> PGSMNELKHAVVPIDLQSFCLEGTLALWVPALENDSEDDSEAIETADDNEKLFKKECVAYDAGVYTSNKSKGSQTLRWSIFQNRTLTIFDVSLNSKKEPLSKFNVKIHFPSNVMKDGVAFSFSEHSDTTIIYAITHARVLYYIRLSKTWFQLPDARLDDDWCLCYRPISFLNQKPDLMAAISTSEICVSFFNGGLTKIILNPKDASHYEQHIDDSSYLFSLKKYLSLQAFKADYRSPNTIISMIFLSTYNVLVMLSLDYKLKVLDLSTNQCVETIELSQTILPLQSFPYLTSDHTTNSFIALYYPDNSHGSFSIYKLNANAHSFKLNVVIEKGIIPPSLPDDEFIPWMLSDFQLISSEGSQSKFLLIIAWKSNLNTVIQKCNLSLDQDESFSCVWSHSLDSFSLIEKTFFDVPTNMSSGDISEIWLQHIFAHNTSIESIQVALLSFQNSSSQVSKNKLDKFGALTISELKNAVLSSIVSTIQIEPNSDLTGYDYYEYKRLLYNEWERFAKLVA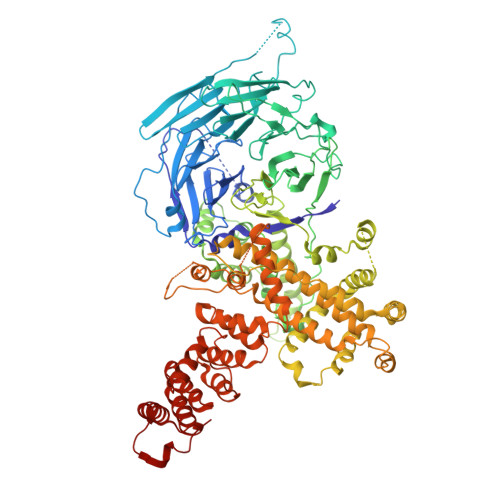YLDHFGDEILSINFDPSNAVTYINYANKVAFIRDPYLIESFDEEPLTKLISSLETDDPSLIEGYQILDLGRSLHSCMSFSTLSEIRYSLRELVQDLPSYSLFDTLWVFYDKHIYPNVDPDYISTLIDTLVSLENPMRDIDSLIQRLRSFDIYNHSAQSPSLFLCASVARVLDSILKKFQVSIEGFIFLLSLITSQQDYELQSKFAGCDKLFLSLLEDWRLVSFLLENSALLLEKFEEEDVDSTNCNLNTMEALASVNTALQFFSALNYSECFSESQISPLHATVISSLSAIFIRDDTENDLVTELVEKLFLFKQYNACMQLIGWLNSDPIAVYLKALIYLKSKEAVKAVRCFKTTSLVLYSHTSQFAVLREFQEIAEKYHHQNLLSCYYLHLSKKLFEESAYIDALEFSLLADASKETDDEDLSIAITHETLKTACAAGKFDAAHVALMVL>GXGTAUACG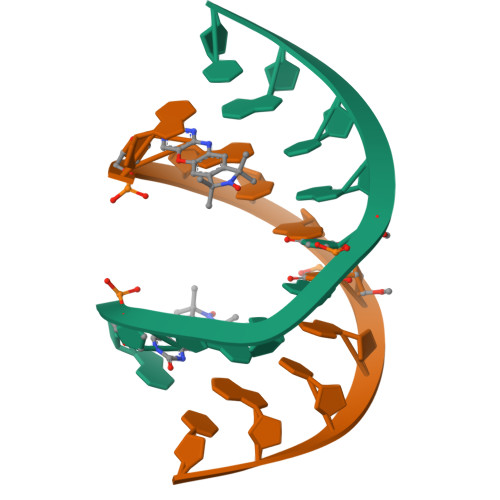C[2x]>[2x]MAKPTVKEIKSLQNFNRIAGVFHLLQMLAVLALANDFALPMTGTYLNGPPGTTFSAPVVILETPVGLAVALFLGLSALFHFIVSSGNFFKRYSAS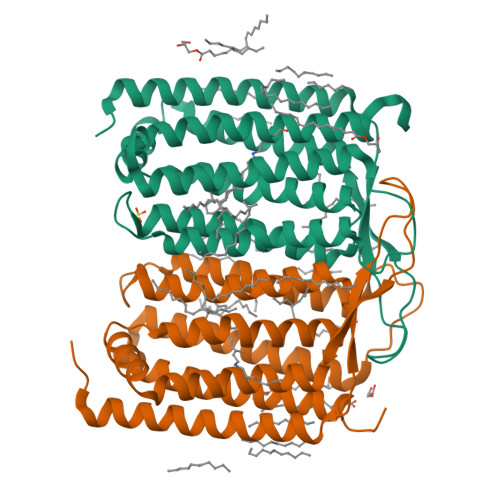LMKNQNIFRWVEYSLSSSVMIVLIAQICGIADIVALLAIFGVNASMILFGWLQEKYTQPKDGDLLPFWFGCIAGIVPWIGLLIYVIAPGSTSDVAVPGFVYGIIISLFLFFNSFALVQYLQYKGKGKWSNYLRGERAYIVLSLVAKSALAWQIFSGTLIPALEHHHHHH> MSSEYAKQLGAKLRAIRTQQGLSLHGVEEKSQGRWK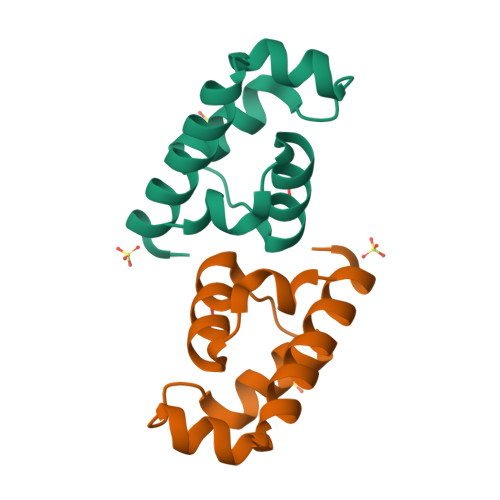AVVVGSYERGDRAVTVQRLAELADFYGVPVQELLP>[4x]MQRGSAYFLRGRARQNLKVLLLYCAFLLVMLLAYASIFRYLMWHLEGRAYSFMAGIYWTITVMTTLGFGDITFESDAGYLFASIVTVSGVIFLDIILPFGFVSMFLAPWIERRLRYHPTIELPDDTRGHILIFGIDPITRTLIRKLESRNHLFVVVTDNYDQALHLEEQEGFKVVYGSPTDAHVLAGLRVAAARSIIANLSDPDNANLCLTVRSLCQTPIIAVVKEPVHGELLRLAGANQVVPLTRILGRYLGIRATTCGALAHILDSFGNLQIAELPVHGTPFAGKTIGESGIRQRTGLSIIGVWERGSLTTPQRETVLTEQSLLVLAGTKSQLAALEYLIGEAPEDELIFIIGHGRIGCAAAAFLDRKPVPFILIDRQESPVCNDHVVVYGDATVGQTLRQAGIDRASGIIVTT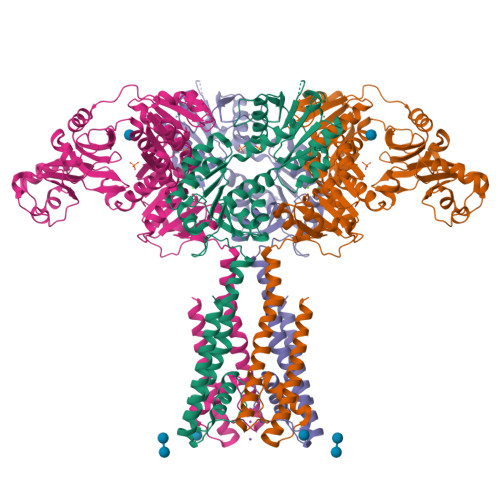NDDSTNIFLTLACRHLHSHIRIVARANGEENVDQLYAAGADFVVSNASVGANILGNLLEHKESAFLSEGMAVFRRPLPPAMAGKTIAETRLRPLTGCSIVAIEAPDRADILISPPPETILAEGARLILIGTSEQEKTFDQTIAARLVPR> MGAIESRKLLASETPVGQFIPYSHHVTDTIISTKNAEYLSVWKIDGRSHQSASEADVFQWIRELNNTLRGISSANLSLWTHIVRRRVYEYPDAEFDNVFCRQLDEKYRESFTGYNLMVNDLYLTVVYRPVSDKVLSFFAKRERETPDQKKHRQESCIKALEDINRTLGQSFKRYGAELLSVYEKGGHAFSAPLEFLARLVNGEHIPMPICRDRFSDYMAVNRPMFSKWGEVGELRSLTGLRRFGMLEIREYDDATEPGQLNVLLESDYEFVLTHSFSVLSRPAAKEYLQRHQKNLIDARDVATDQIE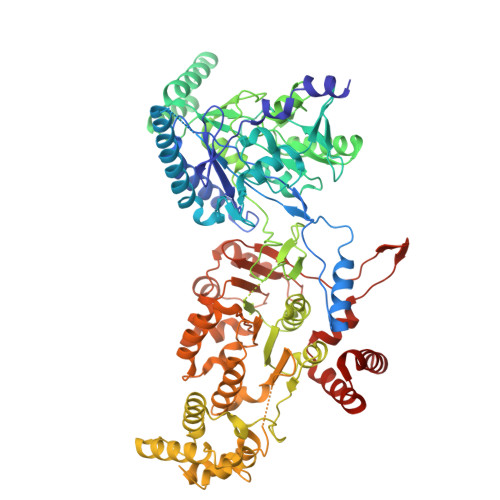EIDEALNQLISGHFVMGEHHCTLTVYGETVQQVRDNLAHASAAMLDVAVLPKPVDLALEAGYWAQLPANWQWRPRPAPITSLNFLSFSPFHNFMSGKPTGNPWGPAVTILKTVSGTPLYFNFHASKEEEDATDKRLLGNTMLIGQSSSGKTVLLGFLLAQAQKFKPTIVAFDKDRGMEISIRAMGGRYLPLKTGEPSGFNPFQLPPTHANLIFLKQFVKKLAAAGGEVTHRDEEEIDQAITAMMSDSIDKSLRRLSLLLQFLPNPRSDDMDARPTVHARLVKWCEGGDYGWLFDNPTDALDLSTHQIYGFDITEFLDNPEARTPVMMYLLYRTESMIDGRRFMYVFDEFWKPLQDEYFEDLAKNKQKTIRKQNGIFVFATQEPSDALESNIAKTLIQQCATYIFLANPKADYEDYTQGFKLTDSEFELVRGLGEFSRRFLIKQGDQSALAEMNLGKFRTIVDGETVERDFDDELLVLSGTPDNAEIAESIIAEVGDDPAVWLPIFLDRVKAERSDV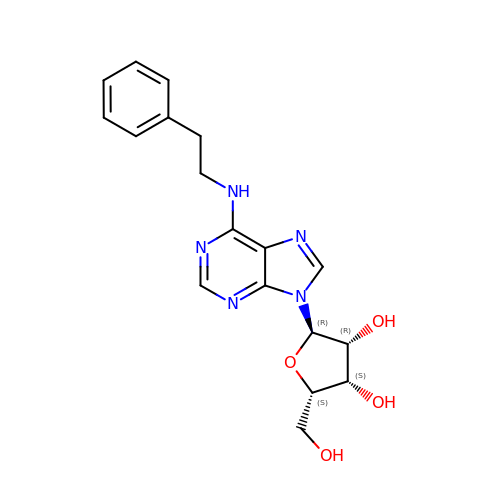9-alpha-L-lyxofuranosyl-N-(2-phenylethyl)-9H-purin-6-amine | C18 H21 N5 O4 | LGZYEDZSPHLISU-KDQZPGIASA-N N,1-dibenzyl-6-[(2-fluorophenyl)sulfonyl]-4,5,6,7-tetrahydro-1H-pyrrolo[2,3-c]pyridine-2-carboxamide | C28 H26 F N3 O3 S | 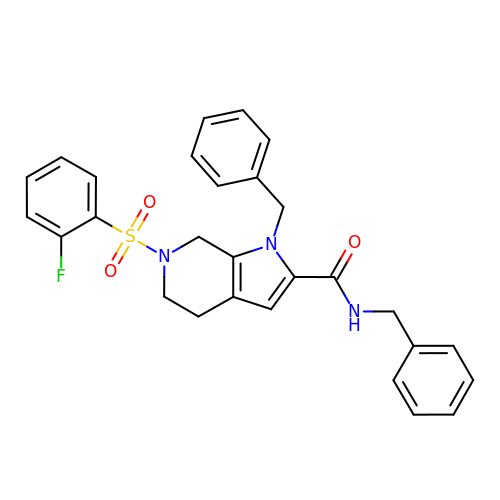RHCKOZJXWTXZPZ-UHFFFAOYSA-N> TNATGERNLALIQEVLEVFPETARKERRKHMMVSDPKMKSVGKCIISNRKSQPGVMTVRGCAYAGSKGVVFGPIKDMAHISHGPVGCGQYSRAGRRNYYTGVSGVDSFGTLNFTSDFQERDIVFGGDKKLSKLIEEMELLFPLTKGITIQSECPVGLIGDDISAVANASSKALDKPVIPVRCEGFRGVSQSLGHHIANDVVRDWILNNREGQPFETTPYDVAIIGDYNIGGDAWASRILLEEMGLRVVAQWSGDGTLVEMENTPFVKLNLVHCYRSMNYIARHMEEKHQIPWMEYNFFGPTKIAESLRKIADQFDDTIRANAEAVIARYEGQMAAIIAKYRPRLEGRKVLLYMGGLRPRHVIGAYEDLGMEIIAAGYEFAHNDDYDRTLPDLKEGTLLFDDASSYELEAFVKALKPDLIGSGIKEKYIFQKMGVPFRQMHSWDYSGPYHGYD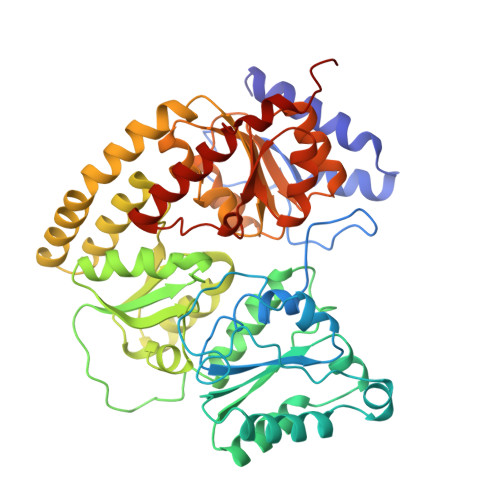GFAIFARDMDMTLNNPAWNELTAPWL>MRGSTDPFELVDIPKISYNPSELSEPRFLEYSNLSDKLHLREAIDKILIPRVVGTTNHSIVREYIVQSLRDLDWDVEVNSFHDHAPIKGKLHFHNIIATLNPNAERYLVLSAHYDSKYMPGVEFLGATDSAVPAAMLLNLAQVLQEQLKPLKKSKLSLMLLFFDGEEAFEEWGPKDSIYGARHLAKKWHHEGKLDRIDMLVLLDLLG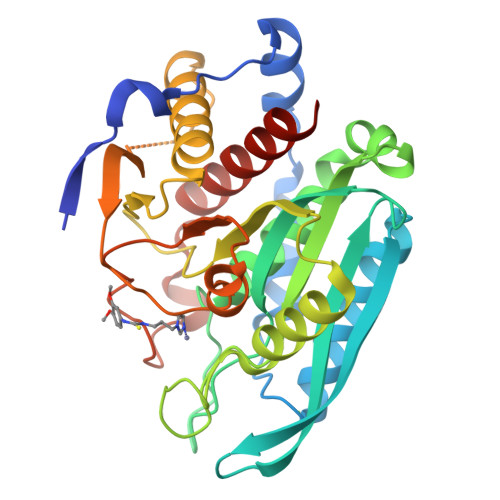APDPAFYSFFENTESWYMRIQSVETRLAKLQLLERYASSGVAQRDPTRYFQSQAMRSSFIEDDHIPFLRRNVPILHLIPVPFPSVWHTPDDNASVIDYATTDNLALIIRLFALEYLLAGTEAK[2x]>MKVAVLPGDGIGPEVTEAALKVLRALDEAEGLGLAYEVFPFGGAAIDAFGEPFPEPTRKGVEEAEAVLLGSVGGPKWDGLPRKIRPETGLLSLRKSQDLFANLRPAKVFPGLERLSPLKEEIARGVDVLIVRELTGGIYFGEPRGMSEAEAWNTERYSKPEVERVARVAFELARKRRKHVVSVDKANVLEVGEFWRKTVEEVGRGYPDVALEHQYVDAMAMHLVRSPARFDVVVTGNIFGDILSDLASVLPGSLGLLPSASLGRGTPVFEPVHGS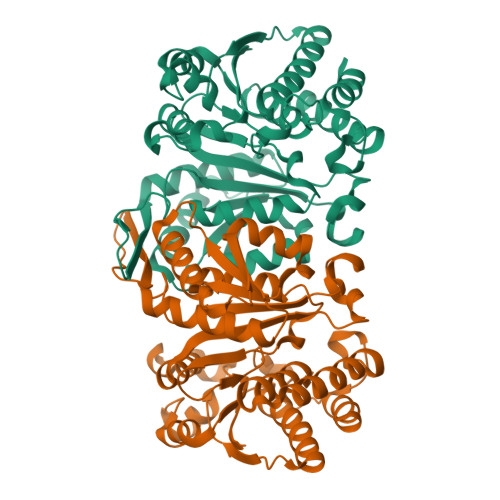APDIAGKGIANPTAAILSAAMMLEHAFGLVELARKVEDAVAKALLETPPPDLGGSAGTEAFTATVEAFTATVGI[2x]>EFQVLFVLTILTLISGTIFYSTVEGLRPIDALYFSVVTLTTVGYGDFSPQTDFGKIFTILYIFIGIGLVFGFIHKLAVNVQLPSILSNLVPR[2x]

The introduction of Asp66Tyr and Asn68Asp mutations in the NaK amino acid sequence causes main-chain conformational changes of the GYG residues in the selectivity filter. This double NaK mutant named NaK2K possesses the conserved amino sequence (TVGYG) found in all potassium ion channels. The NaK channel shares a high amino acid sequence homology and a similar structure with the bacterial KcsA potassium ion channel from S. lividans, but its selectivity filter adopts a different conformation. Both NaK and KcsA are tetrameric ion channels composed of four identical polypeptide chains which form a symmetrical structure. The selectivity filter displays a high selectivity for potassium ions over sodium ions and is formed from four contiguous and chemically equivalent binding sites.

Using much shorter wavelength X-rays (0.97 Å), we were able to collect a dataset to atomic resolution (1.20 Å) for NaK2K, enabling us to reveal in unprecedented detail the protein structure of NaK2K. The overall protein structure of NaK2K remains similar to the previously reported structure (a RMSD of 0.28 Å for all Cα atoms). However, the increased resolution of our structure enabled us to visualize several unseen alternative conformations, such as Phe92, which has an important role in regulating the flow of ions through the selectivity filter. Within the asymmetric unit of the crystal are two identical polypeptide chains (A and B). When the fourfold symmetry of the I4 space group is applied, three additional symmetry-related molecules are generated to form an intact potassium ion channel from each of the two polypeptide chains in the asymmetric unit. In the A polypeptide chain, at the bottom of the selectivity filter on the intracellular side Phe92 is observed in a dual conformation, with the A conformation having a refined occupancy of 68% and the B conformation having a refined occupancy of 32%. In the B polypeptide chain within the unit cell, Phe92 is again in dual conformation, with a refined occupancy of 69% for the A conformation and 31% for the B conformation. The A conformation (68% occupancy) corresponds to an enlarged pore conformation of the ion channel in its open form while the B conformation (32% occupancy) corresponds to a restricted form of the open form of the ion channel. Thus, the dual conformations of Phe92 observed in our structure indicate that in the open form of NaK2K, which is caused by the deletion of the interfacial helix, the two conformations of Phe92 co-occur; one is a restricted pore form which limits ion conductance while the other is an enlarged pore form which is more conducive to ion permeation.> MKVIIIGGETTAYYLARSMLSRKYGVVIINKDRELCEEFAKKLKATIIHGDGSHKEILRDAEVSKNDVVVILTPRDEVNLFIAQLVMKDFGVKRVVSLVNDPGN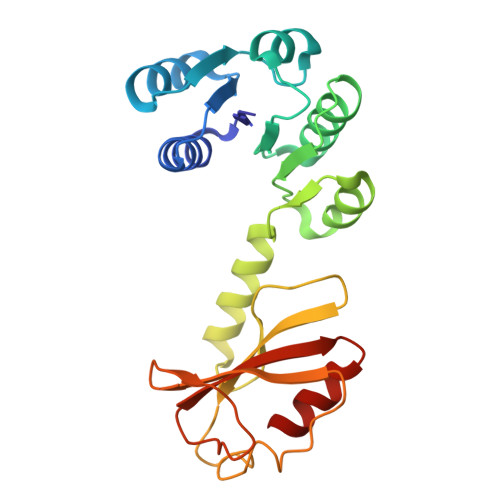MEIFKKMGITTVLNLTTLITNTVEALIFPDEFSSIIPLEQGIEFLSVNVEEDSPVVGKKLKDLPLPRDSIIAAIVRGGVLVVPRGDTEILSGDKLYVIVSAEAKETVEETLLGR>[7x]MEWDSGSDLSADDASSLADDEEGGLFPGGGPI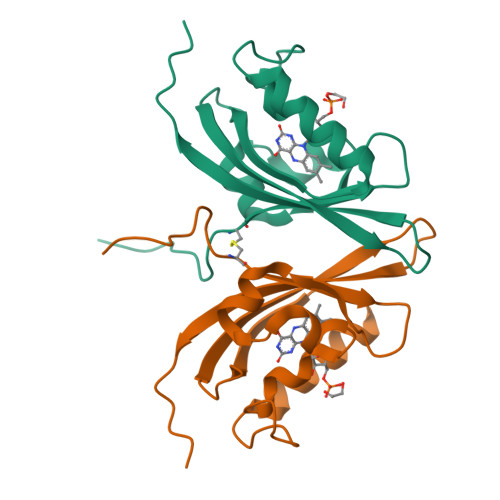PYPVGNLLHTAPCSFVVTDAVEPDQPIIYVNTVFEMVTGYRAEEVLGRNCRFLQCRGPFAKRRHPLVDSMVVSEIRKCIDEGIEFQGELLNFRKDGSPLMNRLRLTPIYGDDDTITHIIGIQFFIETDIDLGPVLGSSTKEKSIDGIYSALAAGERNV> MGAMGKSKAEYYNAWSEWERNAPGGNGEQRGMAVSRLRDALDRQSHELELNNLGLSSLPGIQYLPNVTKLFLNGNKLTDIKPLANLKNLGWLFLDENKVKDLSSLKDLKKLKSLSLEHNGISDINGLVHLPQLESLYLGNNKITDITVLSRLTKLDTLSLEDNQISDIVPLAGLTKLQNLYLSKNHISDLRALAGLKNLDVLELFSQEILNKPINHQSNLVVPNTVKDTDGSLTTPAIISDDGDYEKPNVKWHLPEFTNEVSFIFRQLVNIGGSWAIFSGRVTQPLKEGSENLYFQ

Several viral immune evasion mechanisms have hampered the development of an effective vaccine against HCV, among them the remarkable conformational flexibility within neutralization epitopes in the HCV antigens. Here, we report the design of epitope-focused immunogens displaying two distinct HCV cross-neutralization epitopes. To address these limitations, we generated epitope-focused immunogens based on two antigenic regions including one on HCV E1 (residues 314 to 324) and one on HCV E2 (epitope I). Here, we have demonstrated that small thermally stable protein scaffolds that accurately mimic the structure and specific conformation of two HCV neutralization epitopes in complex with a human bnAb can induce nAbs in the context of a murine and a human antibody repertoire.

Epitope I (residues 412 to 423) is a prime example of such a structural flexibility, as epitope peptides comprising this segment have been crystallized in complex with nAb fragments in three distinct conformations. This suggests that the conformation of this amino acid segment follows an “induced-fit” binding mode to the antibody, and this conformational flexibility could explain the limited immunogenicity to the epitope I observed in patients with HCV. Binding kinetics of E2_EpiI scaffolds E2_S2_1 and E2_S3_3 against Fabs AP33 and HCV1 using sE2 as control are shown. Superposition of AP33 and HCV1 Fab complexes onto the designed E2_S3_3T1 structure revealed steric hindrance of Fab AP33 but not Fab HCV1 with juxtaposed loops. The steric clashes are caused by a variation in the angle of approach of the two Fabs to the epitope, which differs by 22° between HCV1 and AP33 (51). Together with the low thermostability profile of E2_S3 variants, a scaffold size that might hinder the assembly of multivalent NPs for immunization and the apparent limited antibody binding of E2_S3 variants, these results identified E1_S1 and E2_S2_1 as the most promising immunogen candidates.> MEKDLQLRVNEKLDVENILKDLDKYTPKRRGWTWRQPAENLQMGPFIYKDASTPLENSVALPSAKYFGDIDPQPLPVITTEIASGRFEDDIRRMRMAAWHGADHIMVIRTAGQSHYDGLIEGTPQGIGGVPITRKQVRAQRKALDLIEEEVGRPINYHSYVSGVAGPDIAVMFAEEGVNGAHQDPQYNVLYRNINMIRSFIDACESKTIMAWADMAQIDGAHNANATAREAWKVMPELMVQHALNSIFSL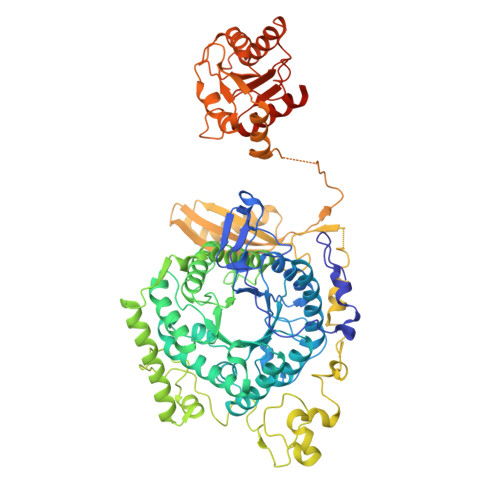KVGMKKSNICLSTVPPTAPPAPSMYLDLPYAVALREMFEGYRMRAQMNTKYMEASTREATVTHVLNLLISKLTRADIQSTITPDEGRNVPWHIYNIEACDTAKQALIGMDGLMDMVQLKREGVLGDTVRELKERAVLFMEEIIEAGGYFNAVEQGFFVDSGYYPERNGDGIARQINGGIGAGTVFERDEDYMAPVTAHFGYNNVKQYDEALVSEPSKLIDGCTLEVPEKIVYIDELDENDNVNVRMEETKEFRHSSMIKPEVEWQADGTVLLTMFLPTSKRVAEFAAIEFAKKMNLEEVEVINREVMQEAEGTRIELKGRVPFSIDINSLVIPPEPEILSEDEIREDIEKTPLKIVAATVGEDEHSVGLREVIDIKHGGIEKYGVEVHYLGTSVPVEKLVDAAIELKADAILASTIISHDDIHYKNMKRIHELAVEKGIRDKIMIGCGGTQVTPEVAVKQGVDAGFGRGSKGIHVATFLVKKRREMREGKSEDPNSSSVDKLAAALEHHHHHH> MVLEVYYTSLRCRCVQESSVFIPRRFIDRIQI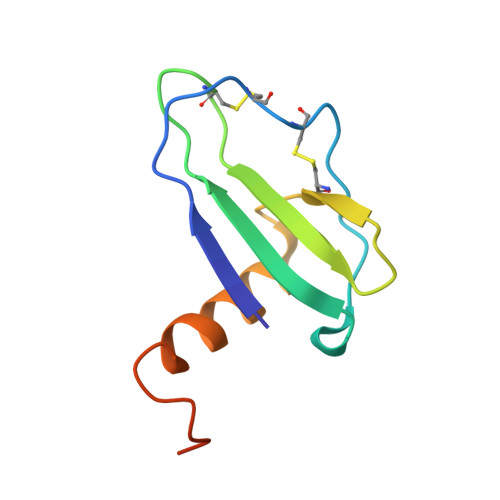LPRGNGCPRKEIIVWKKNKSIVCVDPQAEWIQRMMEVLRKRSSSTLPVPVFKRKIP> MIGVFLRALLIIIYATFVGFIFMGIIRKVTARIHRRIGPPIYQPIIDTLKFFGKKENITHGLIYDFGIIYAVGATILALMFIPLGPISVLRAYGDLILVTFLLEIPMLGIMFAAMSSGNPYAGIGAQRALLTLLAIQVPLGLAIIAVAEYYGTFSTYEIVMAQQKMGWSIFHLPLLLAAIAYDIVLQAMFGKEPFDIMIAPGEISLGPMVEFGGKHMGMLQIQHAMALFAETLFFSNIFLGGGVVTAFGSPLLNTLASLAVLLVKQIAVLLIAIFVGAIFPRFTIDQAAKFYWKWPTIIAAIGAIMAS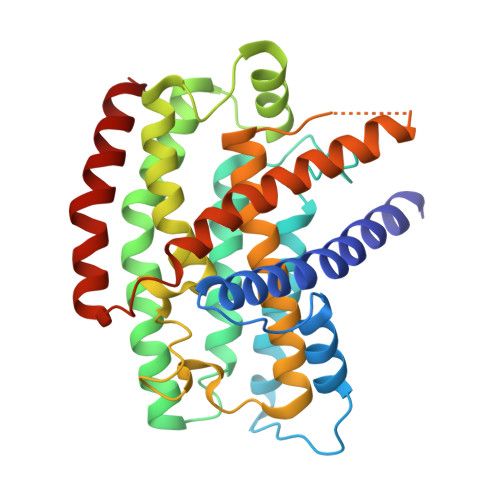L> GSDVNECVTNPCQNDATCLDQI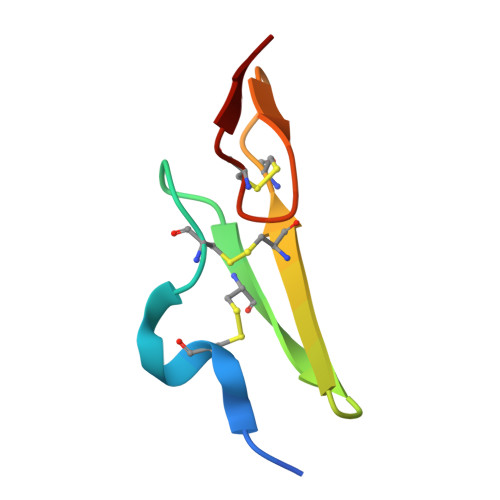GEFQCICMPGYEGVHCEVNT>[2x]GAMGGDGSEFLQRDFSETYERY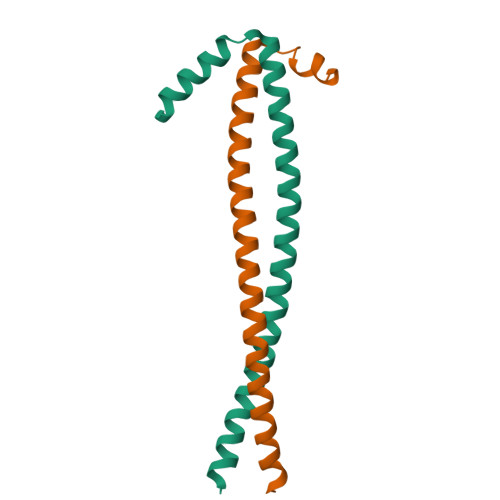HTESLQNMSKQELIKEYLELEKSLSRMEDENNRLRLESKRLDARVRELELELDRLRAENLQLLTENELHRQQERAPLSKFGD>MIRLIFLDIDKTLIPGYEPDPAKPIIEELKDMGFEIIFNSSKTRAEQEYYRKELEVETPFISENGSAIFIPKGYFPFDVKGKEVGNYIVIELGIRVEKIREELKKLENIYGLKYYGNSTKEEIEKFTGMPPELVPLAMEREYSETIFEWSRDGWEEVLVEGGFKVTMGSRFYTVHGNSDKGKAAKILLDFYKRLGQIESYAVGDSYNDFPMFEVVDKVFIVGSLKHK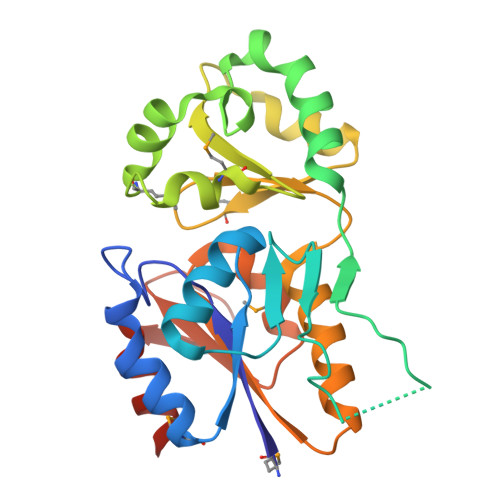KAQNVSSIIDVLEVIKHHHHHH[2x]>MSTSSSSQSLKIGIVGFGNFGQFLAKTMIKQGHTLTATSRSDYSELCLQMGIHFFRDVSAFLTADIDVIVLCTSILSLSEVVGSMPLTSLKRPTLFVDV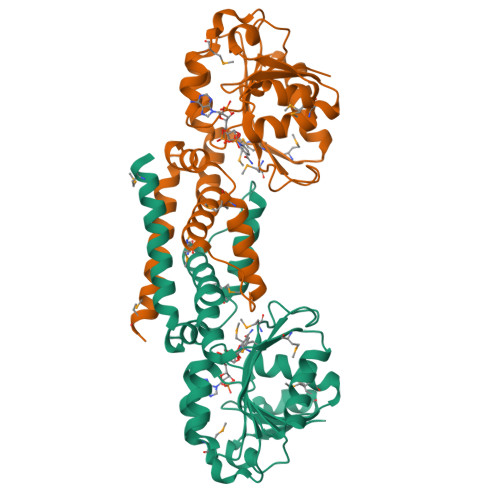LSVKEHPRELLLRELPEDSDILCTHPMFGPQTAKNGWTDHTFMYDKVRIRDEVICSNFIQIFATEGCKMVQMSCEEHDRAAAKSQFITHTIGRTLGEMDIQSTPIDTKGFETLVKLKETMMRNSFDLYSGLFVYNRFARQELENLEHALHKVKETLMIQRTNGEQGHKRTES[2x]> QAGYDLLGDGRPETLWLGIGTLLMLIGTFYFLVRGWGVTDKDAREYYAVTILVPGIASAAYLSMFFGIGLTEVTVGGEMLDIYYARYADWLFTTP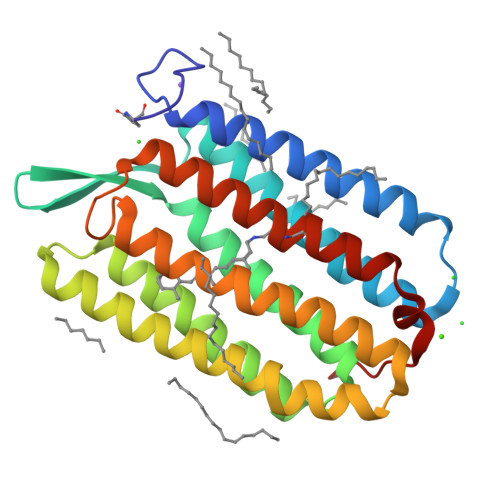LLLLDLALLAKVDRVTIGTLVGVDALMIVTGLIGALSHTAIARYSWWLFSTICMIVVLYFLATSLRSAAKERGPEVASTFNTLTALVLVLWTAYPILWIIGTEGAGVVGLGIETLLFMVLDVTAKVGFGFILLRSRAILGDTEAPE>YHLVDDYGRGNGFFDKFNFFTGDDPTHGYVDYVSRDVAAGAGLIGERDGRTYMGVDFTNPASGRGRRSVRLESKNTYEHGLIVIDLAHMPGSVCGTWPAFWTLGTGDWPYGGAIDIIEGVNDNTFNHMVLHTSDGCTIDNDGFTGNLKTSNCYVYAPGQDANAGCGIEATDPNSYGKGFNSIGGGIYATEITPNG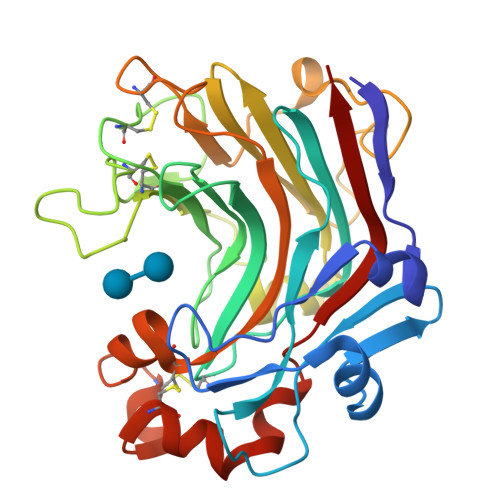ISIWFFPRGSEPGDVLGDNPNPANWDTPAAKFAGGGCDWEGKFNAQRLIFDVTFCGDWAGNVWGIGGCASRAANCVDFVRDNPSAFAESYWLVNSLRVYAP[4x]> MAESVTNPQRPPVIWIGAQECTGCTESLLRATHPTVEN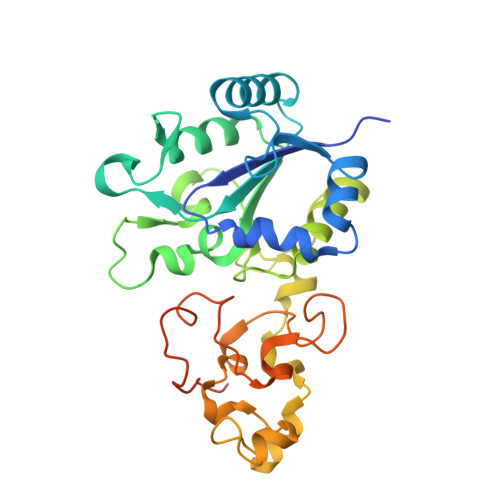LVLETISLEYHEVLSAAFGHQVEENKHNALEKYKGQYVLVVDGSIPLKDNGIYCMVAGEPIVDHIRKAAEGAAAIIAIGSCSAWGGVAAAGVNPTGAVSLQEVLPGKTVINIPGCPPNPHNFLATVAHIITYGKPPKLDDKNRPTFAYGRLIHEHCERRPHFDAGRFAKEFGDEGHREGWCLYHLGCKGPETYGNCSTLQFCDVGGVWPVAIGHPCYGCNEEGIGFHKGIHQLANVENQTPRSQKPDVNAKEGGHHHHHH>[7x]FNAKYVAEATGNFITVMDALKL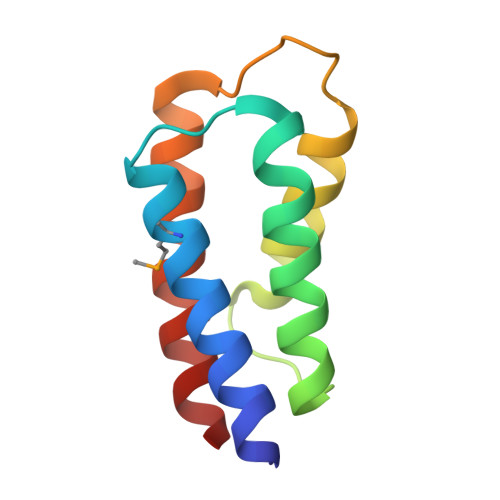NYNAKDQLHPLLAELLISINRVTRDDFENRSKLIDWIVRINKLSIGDTLTETQIRELLFDLELAYKSFYALL> ETPPR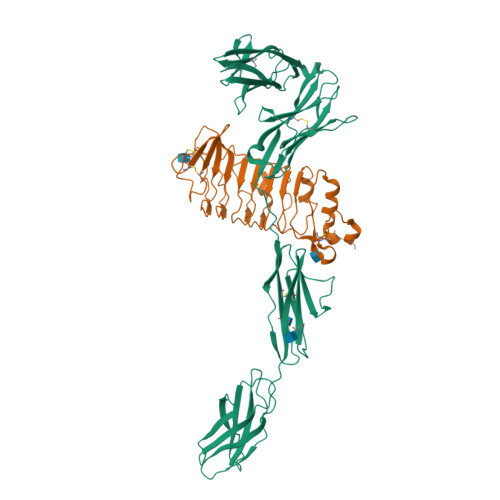FTRTPVDQTGVSGGVASFICQATGDPRPKIVWNKKGKKVSNQRFEVIEFDDGSGSVLRIQPLRTPRDEAIYECVASNNVGEISVSTRLTVLREDQIPRGFPTIDMGPQLKVVERTRTATMLCAASGNPDPEITWFKDFLPVDTSNNNGRIKQLRSESIGGTPIRGALQIEQSEESDQGKYECVATNSAGTRYSAPANLYVRELREVRRVPPRFSIPPTNHEIMPGGSVNITCVAVGSPMPYVKWMLGAEDLTPEDDMPIGRNVLELNDVRQSANYTCVAMSTLGVIEAIAQITVKALPKPPGTPVVTESTATSITLTWDSGNPEPVSYYIIQHKPKNSEEPYKEIDGIATTRYSVAGLSPYSDYEFRVVAVNNIGRGPASEPVLTQKHHHHHH;> MLSGVWFLSVLTVAGILQTESRKTAKDICKIRCLCEEKENVLNINCENKGFTTVSLLQPPQYRIYQLFLNGNLLTRLYPNEFVNYSNAVTLHLGNNGLQEIRPGAFSGLKTLKRLHLNNNKLEVLREDTFLGLESLEYLQADYNYISTIEAGAFSKLNKLKVLILNDNLLLSLPSNVFRFVLLTHLDLRGNRLKVMPFAGVLEHIGGIMEIQLEENPWNCTCDLLPLKAWLDTITVFVGEIVCETPFRLHGKDVTQLTRQDLCPRKHHHHHH>MEEENIVNGDRPRDLVFPGTAGLQLYQSLYKYSYITDGIIDAHTNEVISYAQIFETSCRLAVSLEKYGLDHNNVVAICSENNIHFFGPLIAALYQGIPMATSNDMYTEREMIGHLNISKPCLMFCSKKSLPFILKVQKHLDFLKKVIVIDSMYDINGVECVFSFVSRYTDHAFDPVKFNPKEFDPLERTALIMTSSGTTGLPKGVVISHRSITIRFVHSSDPIYGTRIAPDTSILAIAPFHHAFGLFTALAYFPVGLKIVMVKKFEGEFFLKTIQNYKIASIVVPPPIMVYLAKSPLVDEYNLSSLTEIACGGSPLGRDIADKVAKRLKVHGILQGYGLTETCSALILSPNDRELKKGAIGTPMPYVQVKVIDINTGKALGPREKGEICFKSQMLMKGYHNNPQATRDALDKDGWLHTGDLGYYDEDRFIYVVDRL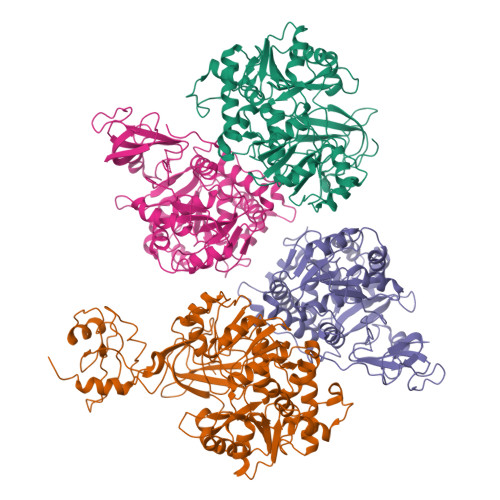KELIKYKGYQVAPAELENLLLQHPNISDAGVIGIPDEFAGQLPSACVVLEPGKTMTEKEVQDYIAELVTTTKHLRGGVVFIDSIPKGPTGKLMRNELRAIFAREQAKSKL[4x]>[2x]SLDLQGSIDYSTLAAGKDFGGVYSSNPLALIRPSGADDVARVLKSACRSSNLTVAARGNGHSINGQAMADGGIVLDMRSTEGNHFKILRINGGDHYADVSGGALWEDILMRCVSEYGLAPRSWTDYLRLTVGGTLSNAGVSGQAFRYGPQSSNVTELDVVTGKGDFLTCSPTQNSDLFFGALGGLGQ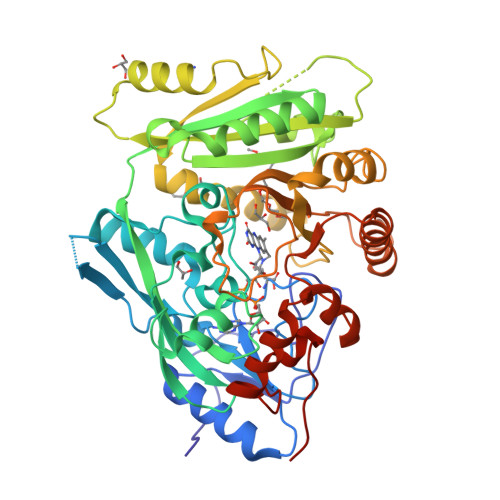FGVITRARIPLEPAPDMVRWIRMVYAEFEDFSRDAEWLVTQPEKESFDYVEGFAFVNSDSPADGWPSVPLNHMMTTPIHSGHQLLYCLELALHFNHSNSSSTVDSVVKRLIGGLRYMKGFKYEVDLSYVEFVMRVKRVEEDARAHGMWDAPHPWLNLFVSKADIAEFDRLIFKGLLHDGVGGPMLVYPLLRSKWDSRSSVVLPEGEDEIFYIVALLRSNPPYPKGPSVDKLVSQNDKIIQSCIQHGLGFKLYLPHYQSQHDWRRHFGDQWSKFVQLKLAFDPMAVLAPGQKIFTRRTKKDPA>[2x]MATEVTFFDELKIDNKVDIIGNNVRGELPN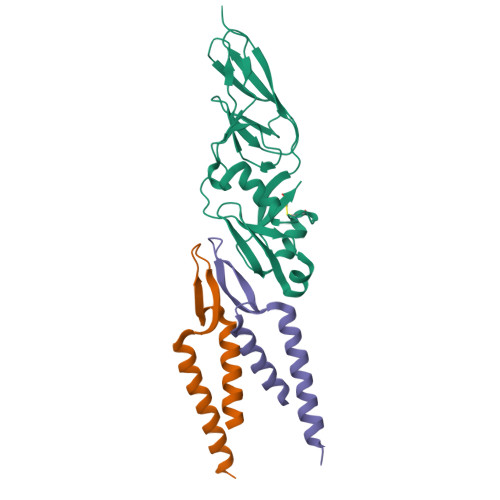IWLQYGQFKLKASGGDGTYSWYSENTSIATVDASGKVTLNGKGSVVIKATSGDKQTVSYTIKAPSYMIKVDKQAYYADAMSICKNLLPSTQTVLSDIYDSWGAANKYSHYSSMNSITAWIKQTSSEQRSGVSSTYNLITQNPLPGVNVNTPNVYAVCVE;>[4x]MDAAASATETATRDQLTKEAFQNPDNQKVNIDELGNAIPSGVLKDDVVANIEEQAKAAGEEAKQQAIENLEHHHHHH> GAMGKSK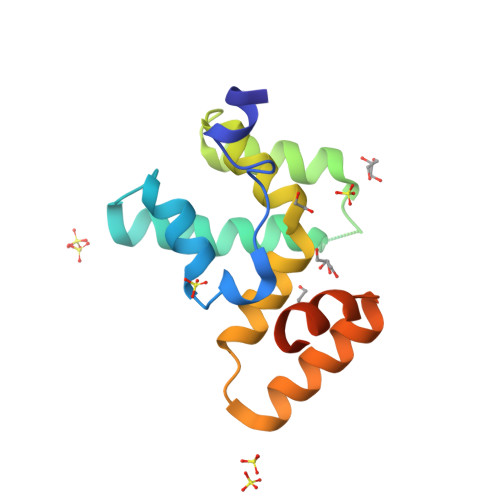SQDKNYVHAREIDAYWLQRQIGRVYPDAHIQHDKTTSALKILSGEPDEPGGDEKQLRDIENDLMELFDYEHHELVQKLIENRDKVVWLTRLARAESREERDTIEREMASEGLRWILDELYGKPKDDQKKPKL> GHMKCPVCHQGEMVSGIKDIPYTFRGRKTVLKGIHGLYCVHCEESIMNKEESDAFMAQVK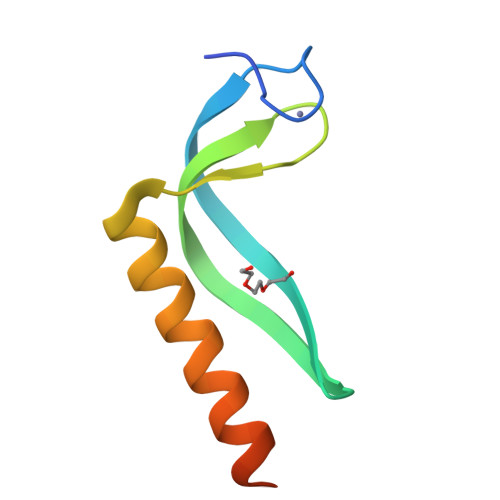AFRASVNAETVAPEFIVK> GSDREYIIKDILDSQEHLLRLIEELLETQKELLEILK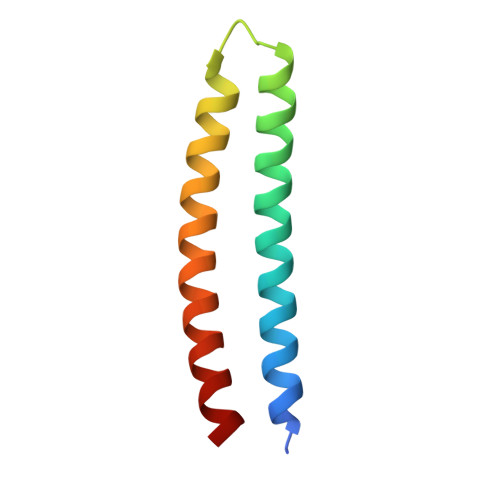RRPDSVERVRELVRRSKEIADEIRRQSDRNVRLLEEVSK> PLGSATITQDTPINQIFTDTALAEKMKTVLGKTNVTDTVSQTDLDQVTTLQADRLGIKSIDGVEYLNNLTQINFSNNQLTDITPLKNLTKLVDILMNNNQIADITPLANLTNLTGLTLFNNQITDIDPLKNLTNLNRLELSSNTISDISALSGLTSLQQLSFGNQVTDLKPLANLTTLERLDISSNKVSDISVLAKLTNLESLIATNNQISDITPLGILTNLDELSLNGNQLKDIGTLASLTNLTDLDLANNQISNLAPLSGLT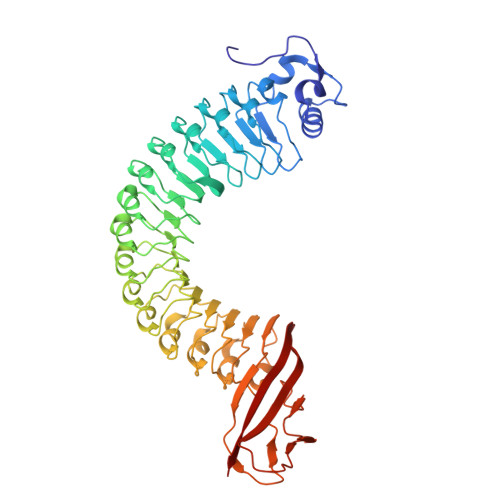KLTELKLGANQISNISPLAGLTALTNLELNENQLEDISPISNLKNLTYLTLYFNNISDISPVSSLTKLQRLFFANNKVSDVSSLANLTNINWLSAGHNQISDLTPLANLTRITQLGLNDQAWTNAPVNYKANVSIPNTVKNVTGALIAPATISDGGSYTEPDITWNLPSYTNEVSYTFSQPVTIGKGTTTFSGTVTQPLKGG>[2x]MADTKAKLTLNGDTAVELDVLKGTLGQDVIDIRTLGSKGVFTFDPGFTSTASCESKITFIDGDEGILLHRGFPIDQLATDSNYLEVCYILLNGEKPTQEQYDEFKTTVTLHTMIHEQITRLFHAFRRDSHPMAVMCGITGALAAFYHDSLDVNNPRHREIAAFRLLSKMPTMAAMCYKYSIGQPFVYPRNDLSYAGNFLNMMFSTPCEPYEVNPILERAMDRILILHADHEQNASTSTVRTAGSSGANP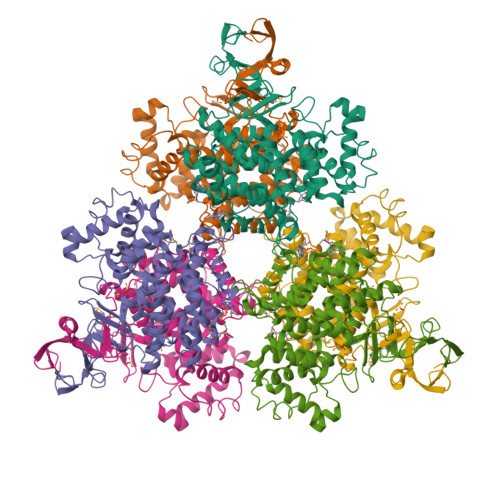FACIAAGIASLWGPAHGGANEAALKMLEEISSVKHIPEFFRRAKDKNDSFRLMGFGHRVYKNYDPRATVMRETCHEVLKELGTKDDLLEVAMELENIALNDPYFIEKKLYPNVDFYSGIILKAMGIPSSMFTVIFAMARTVGWIAHWSEMHSDGMKIARPRQLYTGYEKRDFKSDIKR N-{2-[4-chloro-3-(3-chloro-5-cyanophenoxy)phenyl]ethyl}prop-2-enamide 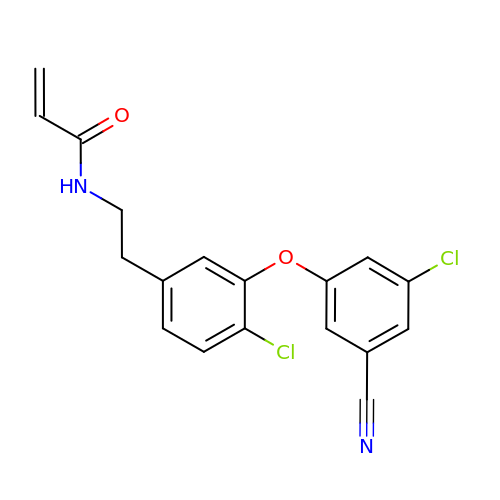| C18 H14 Cl2 N2 O2 | NTQXELUQORLKIR-UHFFFAOYSA-N CISs are macromolecular injection devices with an overall structure that is homologous to the contractile tails of bacteriophages. Their conserved modules include an inner tube, a contractile sheath and a baseplate complex. For firing of the extended apparatus, the baseplate undergoes a conformational change and triggers sheath contraction, which in turn causes the inner tube to be expelled and injected into a target. Here we performed structural and mechanistic studies on a clade Ib CIS gene cluster in the marine bacterium Algoriphagus machipongonensis PR1.

The spike is located below the tube initiator complex and comprises three intertwined copies of Alg8. The N-terminal part of Alg8 forms a gp27-like domain and functions as a 3-to-6-fold symmetry adaptor. The gp27-like domain is followed by the mid β-barrel domain and C-terminal gp5-C-like domain, which are homologous to T4 gp5. Intriguingly, the gp5-C-like and mid β-barrel domains in Alg8 twist an additional 120° around the central axis and are much longer when superposing the gp27-like domains against homologues in PVC/AFP. Interestingly, our symmetry-relaxed map showed an additional prominent density plugged into the tube-exposed cavity of the spike. We identified this density by structural modelling unambiguously as a trimer of the uncharacterized protein Alg6, hereafter referred to as the ‘plug’. Alg6 includes an N-terminal single strand and a C-terminal α-helix, which are linked by a flexible loop. The Alg6 N terminus extends along the inner surface of the Alg8 gp27-like domain, then folds back and forms the C-terminal α-helix. The hydrophobic core of Alg6 contributes to the trimeric assembly, directing the hydrophilic surface to interact with other baseplate components. There are extensive contacts between Alg6, Alg8 and Alg7, suggesting that Alg6 is essential and functions as a nucleus for particle assembly.

>MSTLNKHISIPKDMSSKDDLDFHFLREEGIRYIKELGSNFWTDYNTHDPGITMLEVLCYAISDLGNRINIPIEDLIANEEGGVKGQFYKVQEILPSAPTSELDLRKLFIDIEGIKNCWIKRERVTVFADLKNQKLSYEKTIWEDLKENQKAQFDLKGLYRILVETEDADKVLSESLEKAVFTKFHANRNLCEDLIKVEKVATEPISVCANVEVAPEADEELIHAQILIAIEDYLAPSPRHYSLKQMVDKGYTMDEIFEGPFLENGFIDTVELKASELRKEVRLSDIINIIMSIDGVKIVKEITLGNCDENDGIENNQWVICIPENKKPKLCKKTTINYFKGILPINLNPVRVDNHKSKILASRLENDLKAKDDLEPAIPQGTFADWGEYSSIQHEFPETYGISDIGLPPKLGVKRAVLARQLKGYLLFFDQILASYFEHLSKIKSLLSLDQGPSFTYFTQAIKDIKDVEELFKDPTLLENDEELTKSLIGKLDDTIERRNQLMDHLIARFAENFSSYAFLMKFLYGESTDEIVLQDKQSFLREYKEISRERGEGFNFYEQSNDNLWDTLNVSGAQKRISKLVGVKDYSRRNLSDTAVEIYRYEHVDGNWVYRWRIRDENGKVLLSATTSYPTYNSAGNEMYFAILKILETPLSDLEKLLEVNFRNENEAGSFHFHKAATSNKFSFDIINPVIDSESSSDFIVAKQYTYYPDRTQAVLGAISLLNFIKYTFTEEGIYLVEHILLRPSPLDPEYLAMQTDAGKEYIEGNFLPFCSDDYENCKMIDPYSFRVSIVLPGFTYRFANKDFRDYLENLIREELPAHIVAKICWIGYRKGEEPELFQEDVENPETPIFKENQLEIFEKAYKNYLFELTDIHKRKGFIASMNKYNQVLNEMTSSLTGLHTIYPTGRLYDCEDEEEELDGKLILGKTNLGTL[6x];>[6x]MSENCNHIVTTLKRDGTGRRDLLDPKLAPESVQLQDFELSDWLIFALNFARKIHFFPSDLANEPLGDWRNFFSTIVSDKTLISDIENLDDFEKLRGNIEEFLAAYDQSGKLTPHLTLFVSFLKLLETSKKRFNQLTKRHLDFYYQEILHLEKQALSPDHVFLIFELAKNVSQEKLDEGTEVDGGKDDTGKKNTYLTSFETVLNKTKVGQLKSLYNEISVEKEEIKELNTPISTGTFVMAPMANSFDGLGEDFPKGSEKWWPFGYTKICNASTVLPALPKARLGCSISSKLLKLSEGTRDIILEFTFNKPILPNGEDYTALNKAMSIELTGEKGWIAGLPMTLKSDSGINSGSKKMKLSLTLDSEQPAVVPYQTELHEGSYEVDEPLLRVLFKTNEKEGYNLYRLFNENVLTDLKITVEVSDITSVQLENDLGVLNPQKPFFPFGPRPIKGSSFIVKYPEAMEKPVTAISYQMDYLNLPENLVNHYSAYTIGDDEPLVSDMDYFSVKSFPKSSNDSDQLFSEKSGGGYESDFEFQIENGVWESGLKKELKISLERSFLHEKYAHYFTLVAISKDTDPTIELLPNEPYAPLAENLVLGYTAISSIDFSSSSSENQVSLIHEMPFGFQQVFTPGDTDNSLYLVPDYCHGGELYIGLENGKNLQQVTLLLQFLEGSENPDITDIFTGNQKIKWQYLSQNQWQDFQSGEIIQNQTPRFLKSGIFQFSIPKQANLDNTVLPPGYHWIKASMVKPFDVVSQLINIHAQAVEAVFEDQGSSGNHLEKGLPAETISKLQERLSWIKSIQQPYPSTKGKAQESDEDYYRRVSERLRHKKRAITLWDYEHLILQKFPKVYKVKCLNHTCSSSFQSPGNATLILVPDTVQQSVFDIYQPRVSQGTLNDVAAFVNELNSFHVQAKVINPNYEEVKVDVKVKFREGLDVSFYLTKVKEDIKKFLSPWAYDQESSVEFGVTLHRSQMIHYLEQLTYVDYITDLRLLKRQAGSSPCNPIFIETTEKEYIQPSNPKSILVSAKEHLVTPITQNCSSISLNNEEECQH;>MSEGKLEKLRIVAYKDSKFSDEVENGEFITLLNPEKYKFQYRVEQNEDQASGTSSAPIRFNKILPQTLEFDFLFDRTGVIAGYEVTEDGIINDIDHFKKVVYDYNGEKHKPNYLMITWGSLLFKGYLKEMDIEYKLFRPDGTPIRAMATTKIGEFVEEELRTAQENNQSPDMSHYRTVKEGDTLPLMTYRIYGDSKYYLEVAKANGLTNFRRLKTGTELIFPPLQKQK[6x];>MMEKSKDFLGTGWGFPPEFETSIGQVKTTSGVEDIQKSLEILFSTKIGERIMQPTYGCNLDELLFSPINRTLKTYVIELIKNAILYHEPRIDPEKIDITQGNEIEGELLIHLQYIVRATNSRKNMVYPFYLEEGTNI[6x];>MATYYPPSSFHFLVEFTGIDAKNNDHEFQSVSGLSVDIDTEEFAEGGENRFKHKFPVKTKYPNLVLKRGVLVDSKVISWCRDAIEDFEFKPIDLTVKLLNEEHQPLMTWNVVHAYPVKWSVEDFNAQESKMAIESVELSYNYFKTIV[6x];>[6x]MATYKTPGVYIEEITKFPPSVAQVETAIPAFIGYTQFARTKPSVDSDDLILKPKRISSLLDFTTYYGGAQNEQGITVKLTDTLIEGAENRTINVPEPTFKSPYLMFYSLQMYFANGGGPCYIVSTGVYDDWSDSETPPTINFSDLESGLAVIRKEDEPTLLLFPDATNLPTDDEFYSLYNSALMQCNDLQDRFTILDTYSDQTYNDGVEDLDPIPALRNGINLTKDYLKYGAAYYPFVQTILNYQYSADEIVIQHLSYNPNAIATALDNLNAVNGPTFIDAILDDLRDLSLPDISGEISDAVGFMYDDVDGFDIDGTFTTNSVKVANFASLVESVLSTLNELIDAKEEINKDVNSAIASSEEDNAIKTAISDALDVFNEDFEGADKIESVAKNLSDLLIKIKQADTNTKVENVLSINALNFSAEFEKLLTYDVNTGLTASVTLDLFANIGTRLDDIIAAVSAAEPIDVNNGKLNGRLLSDIEPLDNATYNTILLEINSHKVTLPPSSSMAGAYARVDNDRGVWKSPANIGLNYVSKPSVTVSHEEQESMNVHGTGKSVNAIRSFVGKGTLVWGARTLAGNDNEWRYISVRRFFNMAEESIKKATEQFVFEPNDGNTWVRVRAMIENFLILQWRAGALAGAKPEHAFYVKVGLGQTMTAQDILEGNMNVEIGLAVVRPAEFIILKFSHKMQES;>MSYPLSKFHFSVEWGGTKIGFTEVSGLDLETEIIEYRHGASPEYSKIKMPGMQKFSNITLKRGTFKSDNEYFQWYNTINLNKVERRDLTISLLNEEHEPVVTWKVKNAWPLKVQSTDLKGDGNEVAIESMELAHEGLVIQNE[6x];>MNNSGTIETSQSVDRVTHKILIDGSEIPGTYQVKSIQVTKEVNRIPTARLVILDGDAAERDFKVSNSDHFVPGKEIEITVGYHSDDETIFKGVVIRQNLKIRNNQSILIVESRDMAVKMTLRRKSKYFYELSDSDILEELISNHGLEADVASTENQHTELVQYDVTDWDFMMLRLQANGLLCLVDDGKVSIQKPDLSSEALETVTFGATILEFDAEMDARNQLPKVVSQAWNMSDQELLEKEGVDPSLETNGNISSSDLASLFDQEEEVLRHGGSKKDGSLQEWANAKWTFQQLAKTRGRIKFQGIPTVKPGVNLLLEGVGDRFNGKVFITGVNHQISEGNWTVDAQFGLNPEWFSESESNIHTPPAAGLTAAISGLHVGLVTDLEDPDGEDRIKVKIPIINNEEEGVWCRQAFPDAGNERGITFRPEIEDEVIVGFINEDPNDAVVLGMLHSSANPNPIEASNDNHEKGIQTRSGIKMIFNDEKSILQIETPTGNLVTLDDDAGSITIEDQNGNKTVMDSDGITMESAKDMNLKASGDINLEGTNVNIKANAEFKAEGSAGAEVSTSAVAVLKGSLVQIN[3x];>MPIEIKELHIKITVDDSNNAGRGGASSGEDKQQLVAQCVEQVLDVLKSQKER[3x]> MGSSYHHHHHHSSGENLYFQHMKHGRVFIIKSYSEDDIHRSIKYNIWCSTEHGNKRLDAAYRSMNGKGPVYLLFSVNGSGHFCGVAEMKSAVDYNTCAGVW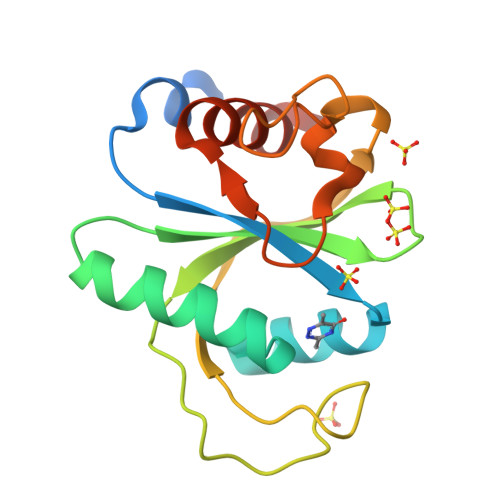SQDKWKGRFDVRWIFVKDVPNSQLRHIRLENNENKPVTNSRDTQEVPLEKAKQVLKIIASYKHTTS> 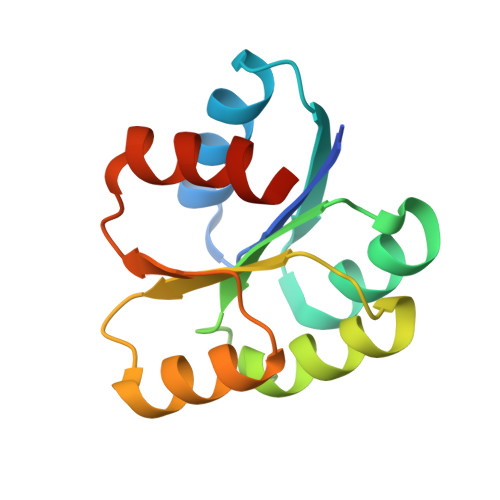GSMMNEKILIVDDQYGIRILLNEVFNKEGYQTFQAANGLQALDIVTKERPDLVLLDMKIPGMDGIEILKRMKVIDENIRVIIMTAYGELDMIQESKELGALTHFAKPFDIDEIRDAVKKYLPLKSN>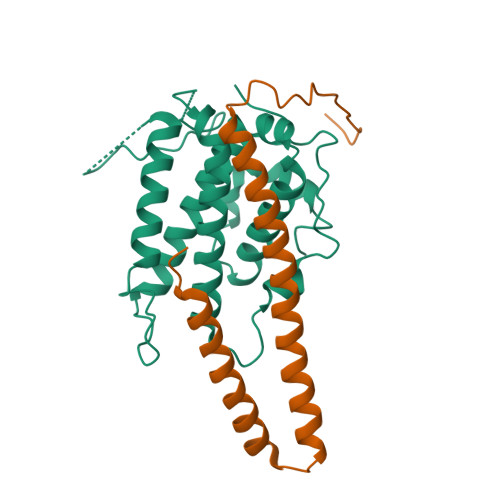 GSLRNKHHSPKRHSQTSFPAQKSTPQSQQLTSTTPQSQQQEASERSESQQIMFLSEPFVRTALVKGSFKTIVQLPKYVDLGEWIALNVFEFFTNLNQFYGVVAEYCTPDACPTMNAGPHTDYLWLDANNRQVSLPASQYIDLALTWINNKVNDKNLFPTKNGLPFPQQFSRDVQRIMVQMFRIFAHIYHHHFDKIVHLSLEAHWNSFFSHFISFAKEFKIIDRKEMAPLLPLIESFEKQGKIIYN;> GSASSPVQSGFNNGTISNYMYFERRPDLLTKGTQDKAAAVKLKIENFYQSSVKYAIERNERRVELETELTSHNWSEERKSRQLSSLGKKESQFLRLRRTRLSLED3-(phenylethynyl)-2-(1H-pyrrol-1-yl)benzoic 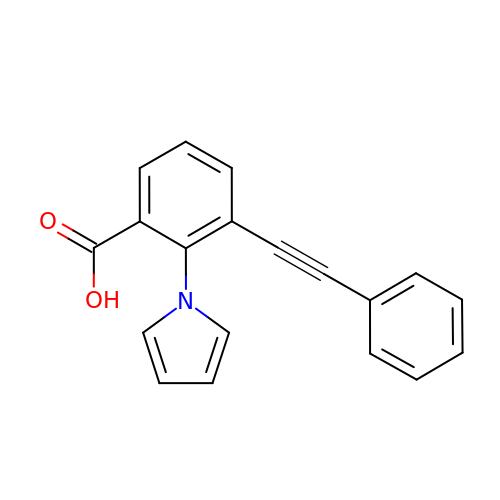acid | C19 H13 N O2 | HJQNYWHFUNEICK-UHFFFAOYSA-N> MDINDDLNINSPVDNKNVVIVRARKTNTFFKAFKVAPNIWVAPERYYGEPLDIAEEYKLDGGIYDSNFLSQDSERENF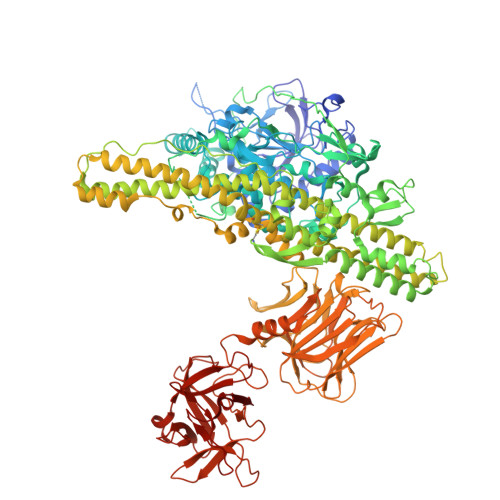LQAIITLLKRINNTISGKQLLSLISTAIPFPYGYVGGGYSSPNIFTFGKTPKSNKKLNSLVTSTIPFPFGGYRETNYIESQNNKNFYASNIVIFGPGSNIVENNVICYKKNDAENGMGTMAEILFQPLLTYKYNKFYIDPAMELTKCLIKSLYFLYGIKPSDDLVVPYRLRTELDNKQFSQLNIIDLLISGGVDLEFINTNPYWFTNSYFSNSIKMFEKYKNIYETEIEGNNAIGNDIKLRLKQKFQNSVQDIWNLNLNYFSKEFNSIIPDRFSNALKHFYRKQYYTMDYGDNYNINGFVNGQINTKLPLSDKNTNIISKPEKVVNLVNANNISLMKSNIYGDGLKGTTEDFYSTYKIPYNEEYEYRFNDSDNFPLNNISIEEVDSIPEIIDINPYKDNSDDLLFTQITSTTEEVITHTALPVNYLQAQIITNENFTLSSDFSKVVSSKDKSLVYSFLDNLMSYLETIKNDGPIDTDKKYYLWLKEVFKNYSFDINLTQEIDSSCGINEVVIWFGKALNILNTSNSFVEEYQNSGPISLISKKDNLSEPNIEIDDIPDSLLGLSFKDLNNKLYEIYSKNRVYFRKIYFNFLDQWWTEYYSQYFELICMAKQSILAQESVVKQIIQNKFTDLSKASIPPDTLKLIKETTEKTFIDLSNESQISMNRVDNFLNKASICVFVEDIYPKFISYMEKYINNINIKTREFIQRCTNINDNEKSILINSYTFKTIDFKFLNIQAIKNFFNSQVEQVMKEMLSPYQLLLFATRGPNSNIIEDISGKNTLIQYTESVELVYGVNGESLYLKSPNETVEFSNNFFTNGLTNNFTICFWLRFTGKDDDKTRLIGNKVNNCGWEIYFEDNGLVFEIIDSNGNQESVYLSNVINNNWYYISISVDRLKDQLLIFINDKNVANVSIEQILNIYSTNVISLVNKNNSIYVEELSVLDKPVASEEVIRNYFSYLDNSYIRDSSKSLLEYNKNYQLYNYVFPETSLYEVNDNNKSYLSLKNTDGINIPSVKFKLINIDESKGYVQKWDECIICVSDGTEKYLDISPENNRIQLVSSKDNAKKITVNTDLFRPDCITFSYNDKYFSLSLRDGDYNWMICNDNNKVPKGAHLWILKS> RSCIDT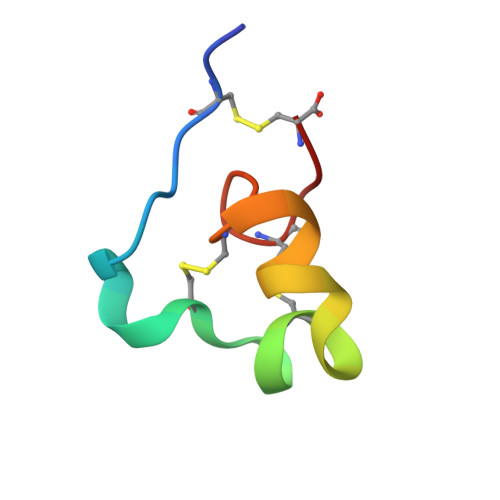IPKSRCTAFQCKHSMKYRLSFCRKTCGTC> GSHMSFLTVPYKLPVSLSVGSCVIIKGTLIDSSINEPQLQVDFYTEMNEDSEIAFHLNVHLGRRVVMNSREFGIWMLEEN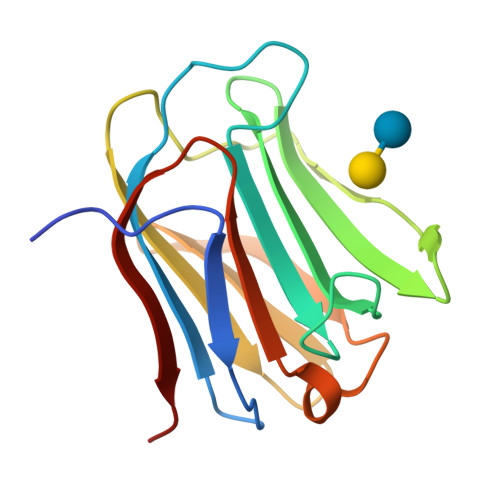LHYVPFEDGKPFDLRIYVCLNEYEVKVNGEYIYAFVHRIPPSYVKMIQVWRDVSLDSVLVNNGRR>[2x]MFKHSTGILSRTVSARSPTLVLRTFTTKAPK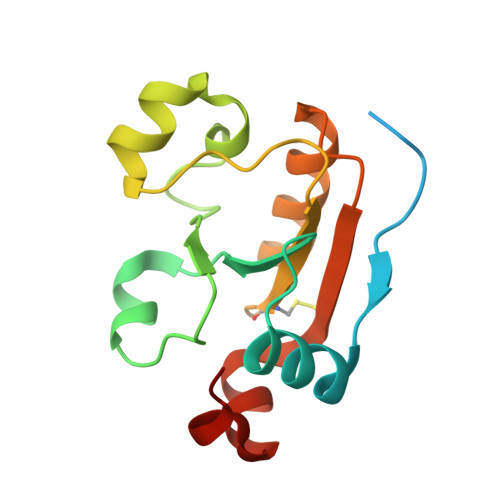IYTFDQVRNLVEHPNDKKLLVDVREPKEVKDYKMPTTINIPVNSAPGALGLPEKEFHKVFQFAKPPHDKELIFLCAKGVRAKTAEELARSYGYENTGIYPGSITEWLAKGGADVKPKK>GPSSPSLLRAIPGIAWIALLLLVIFYVFAVMGTKLFAQSFPEWFGTLGASMYTL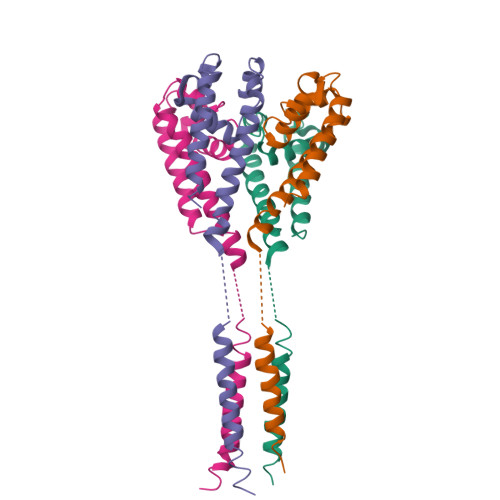FQVMTLESWSMGIARPVIEAYPWAWIYFVSFILVSSFTVLNLFIGIIIESMQSAHWEGGGGGGGEQEQRAHDERLEMLQLIRDLSSKVDRLERRSGKR[4x]>[2x]MGASTRRSSIYRGVTRHRWTGRFEAHLWDKSSWNSIQNKKGKQVYLGAYDSEEAAAHTYDLAALKYWGPDTILNFPAETYTKELEEMQRVTKEEYLASLRRQSSGFSRGVSKYRGVARHHHNGRWEARIGRVFGNKYLYLGTYNTQEEAAAAYDMAAIEYRGANAVTNFDISNYIDRLKKKGVFPFPVNQANHQEGILVEA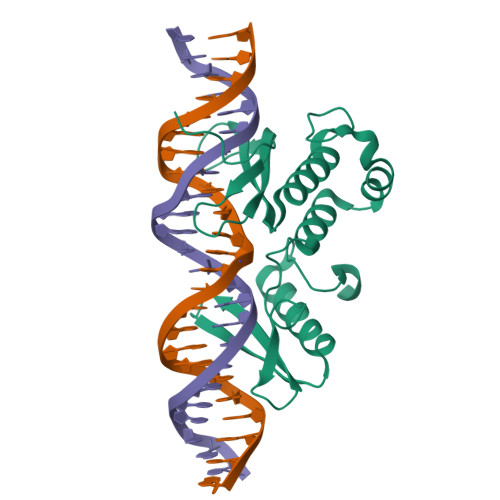KQEVETREAKEEPREEVKQQYVEEPPQEEEEKEEEKAEQQEAEIVGYSEEA> GUU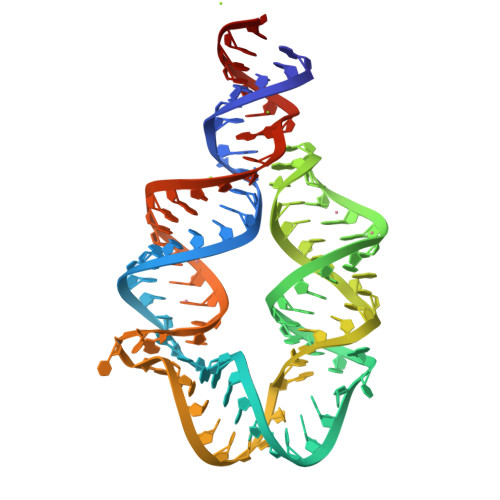GAUAUGGAUUUACUCCGAGGAGACGAACUACCACGAACAGGGGAAACUCUACCCGUGGCGUCUCCGUUUGACGAGUAAGUCCUAAGUCAACA> SYSVGQVAGFAGVTVRTLHHYDDIG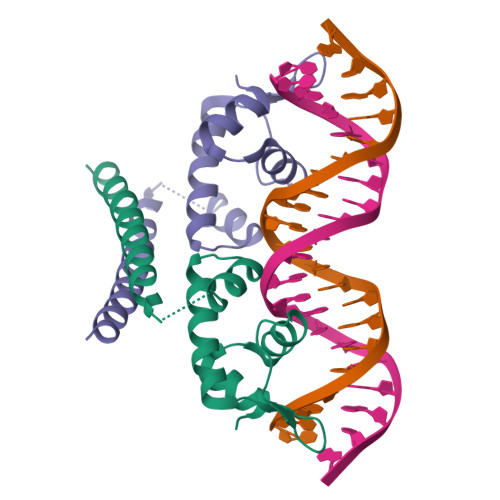LLVPSERSHAGHRRYSDADLDRLQQILFYRELGFPLDEVAALLDDPAADPRAHLRRQHELLSARIGKLQKMAAAVEQAMEARS>[5x]QDMVSPPPPIADEPLTVNTGIYLIECYSLDDKAETFKVNAFLSLSWKDRRLAFDPVRSGVRVKTYEPEAIWIPEIRFVNVENARDADVVDISVSPDGTVQYLERFSARVLSPLDFRRYPFDSQTLHIYLIVRSVDTRNIVLAVDLEKVGKNDDVFLTGWDIESFTAVVKPANFALEDRLESKLDYQLRISRQYFSYIPNIILPMLFILFISWTAFWSTSYEANVTLVVSTLIAHIAFNILVETNLGKTPYMTYTGAIIFMIYLFYFVAVIEVTVQHYLKVESQPARAASITRASRIAFPVVFLLANIILAFLFFGF

During activation of a pentameric ligand-gated ion channel (pLGIC), the binding of agonists promotes the opening of a selective ion conduction pore at a distance of more than 50 Å away from the binding sites. Each subunit consists of a predominantly β-stranded extracellular domain and an α-helical transmembrane pore, which interact via an extended interface. Whereas ELIC forms a cation-selective channel with high conductance that is activated with high efficacy by the primary amines cysteamine, propylamine, and GABA, the cation-selective GLIC is activated by protons and inhibited by bulky positively charged compounds that also act as open channel blockers of the nAChR. Our study has identified a cluster of interacting residues located at the β1-β2 turn, the β6-β7 loop and the pre-M1 region of the extracellular domain, and the M2-M3 loop of the pore that exert a strong influence on channel function.

The equivalent mutation P246G in GLIC results in large rearrangements when compared to WT. The structure determined at 3.2 Å shows a molecule with small differences throughout most of the protein except for the M2-M3 loop and the pore-lining helix M2, which both have undergone major conformational changes. The introduced conformational freedom upon replacement of the restrained amino acid proline with the flexible glycine has resulted in the rearrangement of the M2-M3 loop and the unfolding of the C-terminal part of M2. The remainder of the helix has collapsed towards the pore axis as to maximize the hydrophobic interactions of residues at the extracellular part leading to a structure, which, most probably, prevents the permeation of ions. In contrast to the large conformational change in the extracellular part of the helix, its conformation at the intracellular half remained unchanged. Remarkably, this pore conformation is very similar to structures of GLIC obtained from cysteine crosslinking of residues at the domain interface, which were previously assigned to a locally closed conformation of the ion conduction path, the structures of two nonactivating mutants in the M2-M3 loop and a recent structure of GLIC at neutral pH. In this locally closed conformation, an interaction of a histidine residue in the pore-forming helix M2 with the backbone of the neighboring helix M3 established in the low pH crystal structure of GLIC is broken. When studied by two-electrode voltage clamp electrophysiology, the GLIC mutant P246G shows dose-dependent channel activation with an EC50 that is shifted by 0.5 pH units towards higher proton concentrations. Another distinct nonconducting conformation of the pore region was observed in a high pH crystal form of GLIC and in several mutants of the same channel, including the structure of the mutant P246G determined in this study. Thus, to our surprise, the mutation of a conserved proline in the M2-M3 loop to glycine still promotes activation in both channels, ELIC and GLIC.> MSHLAELVANAAAAINQASDVAALDNVRVEYLGKKGHLTLQMTTLRDLPPEERPAAGAVINAAKEQVQQALNARKAELESAALNARLAAETIDISLPGRRIENGGLHPVTRTIDRIESFFGELGFTVATGPEIEDDYHNFDALNIPGHHPARADHDTFWFDATRLLRT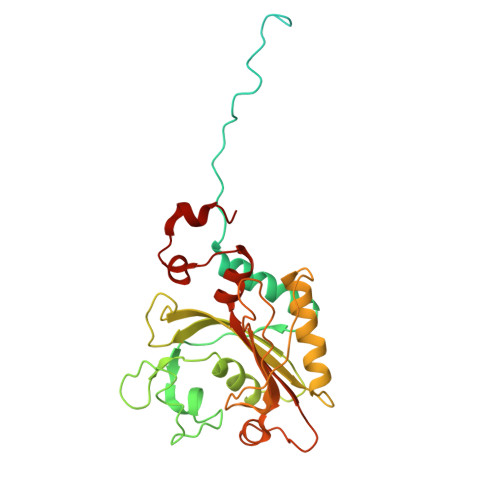QTSGVQIRTMKAQQPPIRIIAPGRVYRNDYDQTHTPMFHQMEGLIVDTNISFTNLKGTLHDFLRNFFEEDLQIRFRPSYFPFTEPSAEVDVMGKNGKWLEVLGCGMVHPNVLRNVGIDPEIYSGFAFGMGMERLTMLRYGVTDLRSFFENDLRFLKQFK> SELDAKLNKLGVDRIAISPYKQWTRGYMEPGNIGNGYVTGLKVDAGV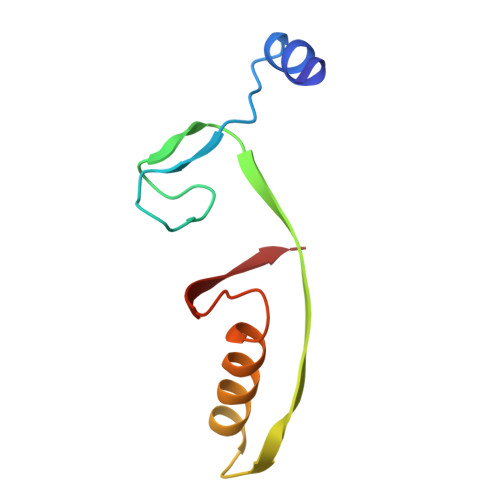RDKSDNNVLDGIVSYDRAETKNAYIGQINMTTAS(2~{S})-2-azanyl-4-[[(2~{S},3~{S},4~{R},5~{R})-5-[4-azanyl-5-(2-quinolin-3-ylethynyl)pyrrolo[2,3-d]pyrimidin-7-yl]-3,4-bis(oxidanyl)oxolan-2-yl]methylsulfanyl]butanoic acid | C26 H26 N6 O5 S | 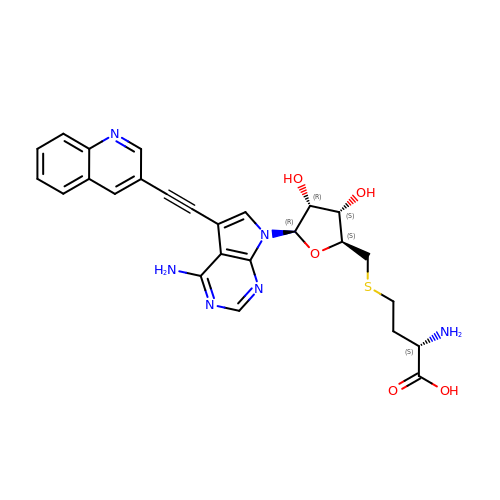SPMFBZXXQBXKFX-LUOSIZPJSA-N> 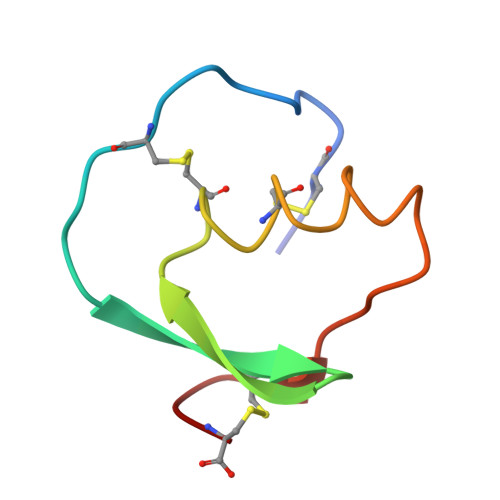VDCSEYPKPACTQEYRPLCGSDNKTYGNKCNFCNAVVESNGTLTLSHFGKC>[2x]EVEV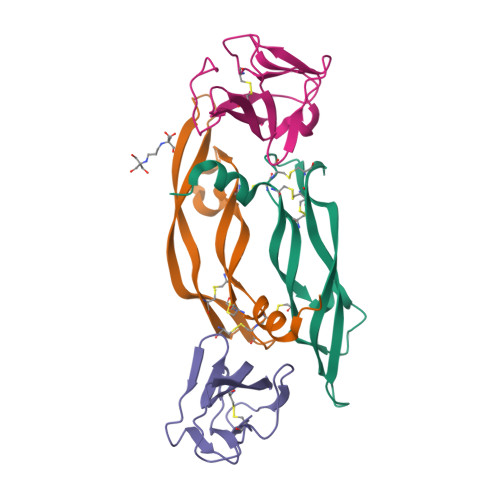VPFQEVWGRSYCRALERLVDVVSEYPSEVEHMFSPSCVSLLRCTGCCGDENLHCVPVETANVTMQLLKIRSGDRPSYVELTFSQHVRCECRPLREKM;>DTGRPFVEMYSEIPEIIHMTEGRELVIPCRVTSPNITVTLKKFPLDTLIPDGKRIIWDSRKGFIISNATYKEIGLLTCEATVNGHLYKTNYLTHRQTNTI[2x]> MTVSTPPSIATGNAPSPDYRVEILSESLPFIQKFRGKTIVVKYGGAAMTSPELKSSVVSDLVLLACVGLRPILVHGGGPDINRYLKQLNIPAEFRDGLRVTDATTMEIVSMVLVGKVNKNLVSLINAAGATAVGLSGHDGRLLTARPVPNSAQLGFVGEVARVDPSVLRPLVDYGYIPVIASVAADDSGQAYNINADTVAGELAAALGAEKLILLTDVAGILENKEDPSSLIKEIDIKGVKK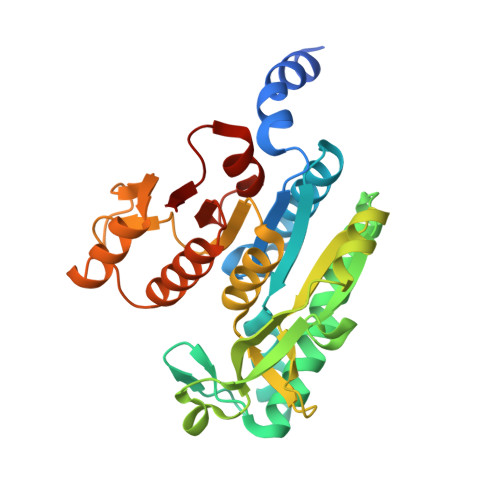MIEDGKVAGGMIPKVKCCIRSLAQGVKTASIIDGRRQHSLLHEIMSDEGAGTMITG Listeria monocytogenes is a pathogenic bacterium that produces flagella, the locomotory organelles, in a temperature-dependent manner. DegU transcriptionally activates the expression of GmaR and flagellar proteins by binding the operator DNA in the fliN-gmaR promoter as a response regulator of a two-component regulatory system. lmDegU contains an N-terminal receiver domain (RD; residues 1–143) and a C-terminal DNA-binding domain (DBD; residues 159–228), which are connected by a 15-residue linker (residues 144–158). Therefore, we conclude that DegU is a noncanonical response regulator that is constitutively active irrespective of phosphorylation.

The crystal structure of lmDegUDBD was determined by molecular replacement and was refined to an Rfree value of 25.3% for the X-ray diffraction data with a resolution of up to 2.39 Å. The asymmetric unit of the lmDegUDBD crystal contains two lmDegUDBD chains (chains A and B), which have essentially identical structures with a root-mean-square deviation value of 0.50 Å. lmDegUDBD adopts a one-domain structure with a tetrahelical helix-turn-helix (HTH) motif as observed for a LuxR-type DNA-binding HTH domain that belongs to the GerE (PF00196) family in the Pfam database. The lmDegUDBD structure consists of four α-helices (α7, α8, α9, and α10), and the two adjacent helices are linked by a 3–4 residue loop. In the lmDegUDBD structure, the α9 helix is the most elongated helix with 15 residues and forms a base frame that supports the other three shorter α-helices. The α9 helix is defined as a recognition helix, which has been shown to be required for dsDNA binding in GerE family members. The dimerization interface of lmDegUDBD (buried surface area, ~ 500 Å2) is mainly located at the α10 helix with additional contributions from the C-terminal region of the α7 helix and the α7-α8 and α9-α10 loops. The α10 helix is parallelly aligned with its equivalent helix from the dimerization partner (α10′; the primer denotes the second lmDegUDBD chain in the dimer structure) and is responsible for ~ 64% of the dimerization interface. To be consistent with the dsDNA-binding ability of lmDegUDBD, the lmDegUDBD dimer structure displays a continuous positive patch that is electrostatically complementary to the negatively charged dsDNA. Each of the three lmDegUDBD mutants (lmDegUDBDR168A, lmDegUDBDN198A, and lmDegUDBDR212A) exhibited lower dsDNA-binding affinity in the FP assay than lmDegUDBD, indicating that the continuous positive patch of the lmDegUDBD dimer covering the R168, R212, and N198 residues mediates dsDNA recognition.

>GSAKDPKMPLHILTHRECEVLQLLTDGKSNRGIGETLFISEKTVKNHVSSILQKMKVNDRTQAVVTAIKHGWVYIR[2x]>MTKKGDTYNEAWVKDTNGFDILMGQFAHNIENIWGFKEVVIAGPKDYVKYTDQYQTRSHINFDDGTITIETIAGTEPAAHLRRAIIKTLLMGDDPSSVDLYSDVDDITISKEPFLYGQVVDNTGQPIRWEGRASNFADYLLKNRLKSRSNGLRIIYSVTINMVPNHLDKRAHKYLGMVRQASRKYGVDESLILAIMQTQSSFNPYAVSRSDALGLMQVVQHTAGKDVFRSQGKSGTPSRSFLFDPASNIDTGTAYLAMLNNVYLGGIDNPTSRRYAVITAYNGGAGSVLRVFSNDKIQAANIIN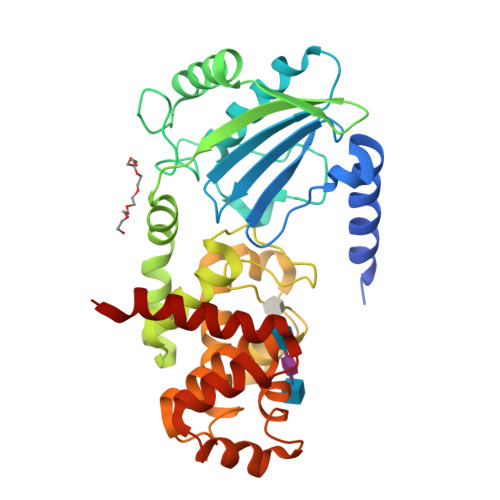TMTPGDVYQTLTTRHPSAESRRYLYKVNTAQKSYRRR[2x]>[7x]GGVLVAQDYRAGSFIELLRNRMALAGVGVRILQGLTG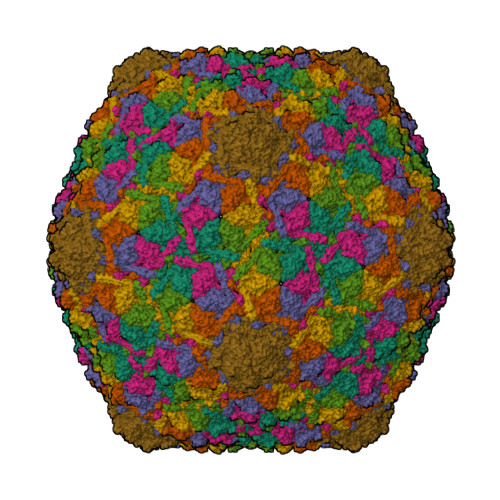NVDIPKRTGASTMYFVDEDVDVTESDGAFGLVGMTPHTAGVATAITRRMMQQGSPDIEALVRDDLLTSLTLGLDKTALVGHSSPSAPNGVRDLVIGDALPFTGPFATFEELVDLETAVASANADVDSMAYIYNAATSGHFKKTLEFAGVSGTIERGGQVNGYNRVKSNQITTAGEVAFGNWSDVVIGMWSGLDLRVDTSTKAASDGKVLRVFTDIDVALRNVESIKWGVPA>FPGCDYEHWLIVMDKPGGEGATKQQMIDCYIQTLAKVVGSEEEAKKRIYNVSCERYLGFGCEID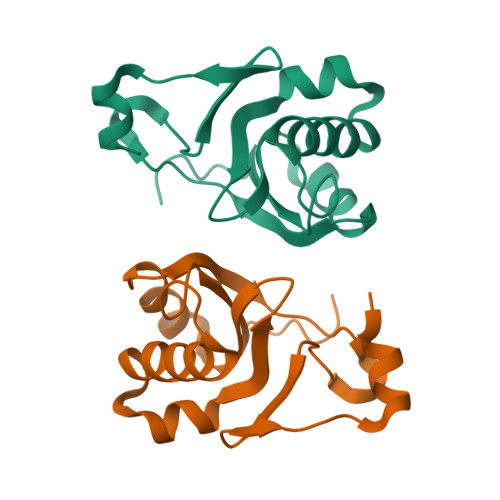EETSTKLEGLPGVLFVLPDSYVDPENKDYGAELFVNGEIVQRSPERQRRVEP[2x]>GSPASGTSLSAAIHRTQLWFHGRISREESQRLIGQQGLVDGLFLVRESQRNPQGFVLSLCHLQKVKHYLILPSEEEGRLYFSMDDGQTRFT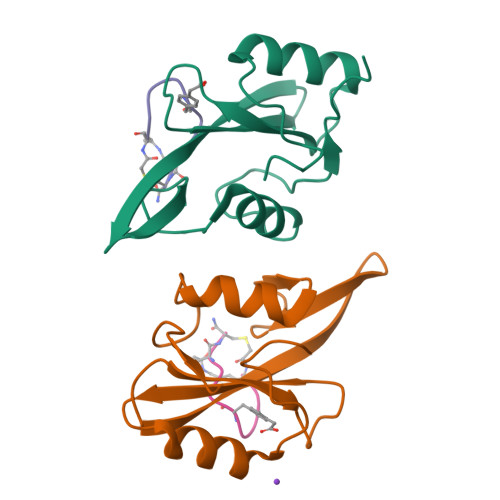DLLQLVEFHQLNRGILPCLLRHCCTRVAL[4x];>[4x]KFEGFDNEX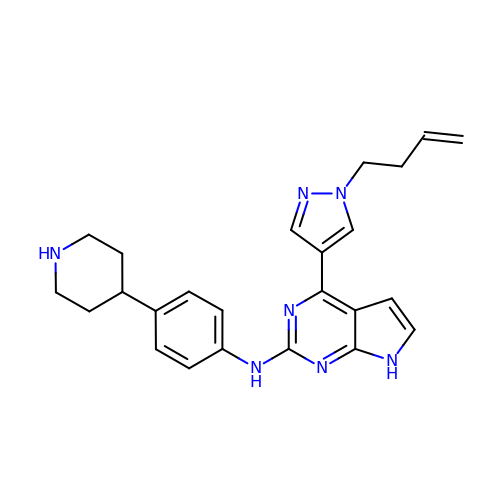4-[1-(but-3-en-1-yl)-1H-pyrazol-4-yl]-N-[4-(piperidin-4-yl)phenyl]-7H-pyrrolo[2,3-d]pyrimidin-2-amine | C24 H27 N7 | OZUDWDBQZJPKOG-UHFFFAOYSA-N> TAVVT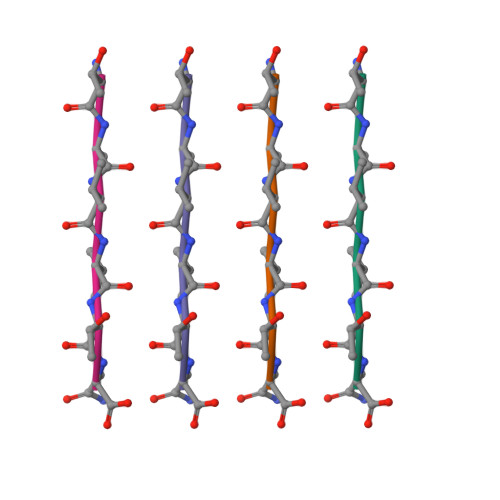N>[3x]PPGPPGPPGPPGLPGLPGP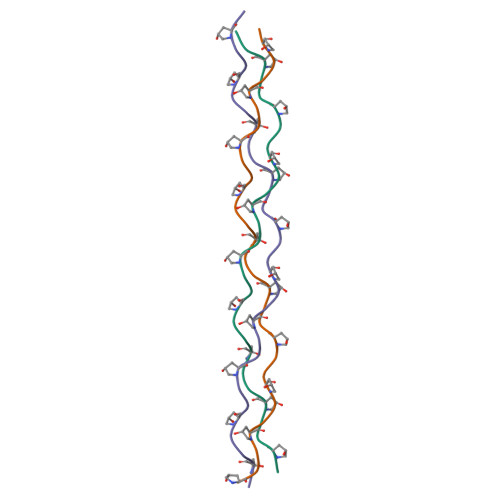PGPPGPPGPPG> GENFMDIECFMVLNPSQQLAIAVLSLTLGTFTVLENLLVLCVILHSRSLRCRPSYLFIGSLAVADLLGSVIFVYSFIDFHVFHRKDSRNVFLFKLGGVTASFTASVGSLFLAAIDRYISIHRPLAYKRIVTRPKAVVAFCL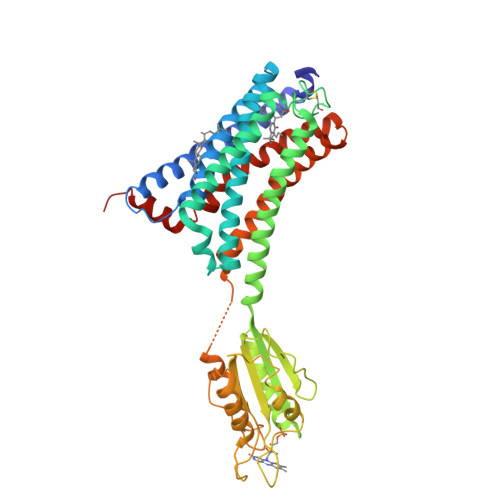MWTIAIVIAVLPLLGWNCEKLQSVCSDIFPHIDKTYLMFWIGVVSVLLLFIVYAYMYILWKAHSHAVAKALIVYGSTTGNTEYTAETIARELADAGYEVDSRDAASVEAGGLFEGFDLVLLGCSTWGDDSIELQDDFIPLFDSLEETGAQGRKVACFGCGDSSWEYFCGAVDAIEEKLKNLGAEIVQDGLRIDGDPRAARDDIVGWAHDVRGAIPDQARMDIELAKTLVLILVVLIICWGPLLAIMVYDVFGKMNKLIKTVFAFCSMLCLLNSTVNPIIYALRSKDLRHAFRSMFPS Here, we report cryo-EM structures that reveal the molecular architecture of the Trypanosoma brucei CBC (TbCBC) complex. We confirm TbCBP20 as the cap-binding subunit and identify TbCBP110 as the homolog of opisthokont CBP80, despite their poor sequence conservation. TbCBP20 and TbCBP110 form the cap-binding core module, which can bind SL RNA independent of the cap4 modifications that are unique to kinetoplastids. TbCBP30 comprises mostly intrinsically unfolded regions and bridges the TbCBP20-TbCBP110 core to the TbCBP66 subunit, which contains an additional SL RNA interaction site with specificity for double-strand RNA.

To gain insight into the architecture of trypanosomatid CBC, we generated a cryo-EM structure of the TbCBC tetramer. Since an affinity assay indicated the ability of the tetramer and dimer to interact with the m7GMP of the RNA 5’-cap, we included the commercially available m7GpppA in our cryo-EM grid preparations. The cryo-EM reconstruction extended to a resolution of 2.4 Å but accounted for only 48% of the residues in the complex. Although most of TbCBP20, TbCBP110, and an N-terminal portion of TbCBP30 could be modeled into the coulomb density, the C-terminal domain of TbCBP20, large parts of TbCBP30, and the entire TbCBP66 were absent. The radius of gyration of 6.15 ± 0.28 nm indicated the presence of the intact tetrameric complex, but the Kratky plot suggested disorder and/or flexible portions of the complex. The reconstructed and modeled portions of the tetrameric complex comprise mainly the large, exclusively α-helical TbCBP110 subunit. At a concave surface of TbCBP110, the smaller TbCBP20 subunit is bound. The N-terminal domain and the central RNA recognition motif (RNP) of TbCBP20 are well-ordered, but the C-terminal domain of TbCBP20 is not resolved indicating its flexibility. The m7GMP portion of the cap-analog is coordinated by TbCBP20. An N-terminal peptide of TbCBP30 (residues R33-I82) is bound in the cleft formed between TbCBP20 and TbCBP110 and the protein continues by forming a large loop across the adjacent surface of TbCBP110.

> HHHHHHHHPPSGADPMYAMPGNSGDLQCDDGKKRHIPPLSLLLSGYGSSEGRELDTSYTPKQWLWFLYVTSWARPFFTYASSGGASEATEGSSDNRSGSAYWGRLSFDELLKLSGSPIPPAMVSLWMGLCMPTDDVVQELRIMTEGKAEGRQRIYPFLPRVAESTFGRALRSLAVRQHISSWMPSHAGDVCAALDVLVRDTLEVIQNSADVRKTARVRCEERDASGEEALEGAFRSMLSASTTAPKVVEATTYRPLFDVKASIPEGGTAQVLIRVANAARLFAALSVEAFGRVKSECAVLLLAHINQRDAPEHVDARAYGVVTGVVEYAMAYRYCRDDGTGRCPLTCAALLLHRLVELQGIVEKDTAAGDRCMGMAVSASRFANMTVACIQELLFCVVAGDTVRWHREHQPDGVSVCPTAARTLTLHETDCLLQVFIPALLQQVGFEWPWSESLRHAKMLDRARTQHIVMEDGVRLDSRSVFEELLVSVARRTYGLRLRAILPQSFDVIAENIFVSIHDVPNEGKSSGGNPEKVADNSSSRFALPLYYRTAGEVLLEYFDRCGPSGITAEETERVLRRATDVQPMVVQLQALGGDTNGGITDCVSYCGELSRTVYFSAREKERLLQRYRCEVLLASLVVYTQLRTVSVVQQLTRQLAPLFEQLLLPLAHERTLSRCPVIASRKGDGVDDNGTPLVDLTPEFKMLVDEIHYEFYPLEWVPEAVDAHIRQECGVREKEGAPYHEGGNGPPCFAQYSLFAAIAHQFGLVLEGNPRGFRGGDGSSSEVRTKAYRFFTLMLLNNLGDAVSSSCELDGAAALAATRRVKDCQDGSENCKQRQAAVRQRGGASFHSVVSACDVVVTMTQCLLPAHLSSHPRMATTGSMSNEWMRRVGEWTRSAYSKYTAYQQQVHGLDLPVPLISLYNSLTFDSVPLARETIRAVRSRLLEKMSVVTASPPGDVETAGKQLLEQHLSSLTVTLTAVGLLPLCVRGGSHVPCATQLLWASPFFSHELLHCGRYEVSV;> MAEYLIDLTPRMAYVDRHELLRSLLTEKEFIERRQEQLNKSTTVYVGNLSFYTTEDQIWEHFSRCGHIRDLVMGLSEVTRTPCGFCFVVFESQDGAMSAVIDLHGTLLDDRVITVSWDVGCDHTRRWGRGAHGGQVVDGVRQNLDSARGGLGVLRREELGVGAAVAEDQLVHYTWIPPRRVEKRGRS;> MRRGSGFVHLNTPAAISYSPGQQVSLSDLRQKRRREECVVLPPIMTVWRSAFSQYTKMWGLTKFAGDIEAEREGEGPILPPIREETVVKSTTHSFKGKSTTVAAAVATPPGEKGIEIVSHHKLCGKQRFVYPDHDGVLSSGIVPKVVISKEEEEEMEANKKYYISPQEMTEEERNAFEELDAMWKSYARGRSEQGARHRAFAGTVTPGDAMTEVEEETGNNRGNARRRLESHTPRQHPQESAAEGNSVAHNTEEALDDALRLIDELLEFN>MNSTYSRDQIMSNYLPVIGITMGDAAGVGAEVVVKSLAHASVYAQCRPLVIGDAKRLERANQIVGGEMKIRRIEDASEARYEQGTIDCIDLGLIPDDLPFGQLSAIAGDAAYQYIKRAVELAQSGKIDAICTAPLNKEALHAGGHKYPGHTEMLAHLTGVDEVSMMLVAPQLRVIHVTTHIGIIDAIRKIEPGLVQRTIERGNATLVKAGIERPRIGVCGINPHAGENGLFGYGEEEEKIIPAVTLLQERGLDVTGPLPADTLFFRAGR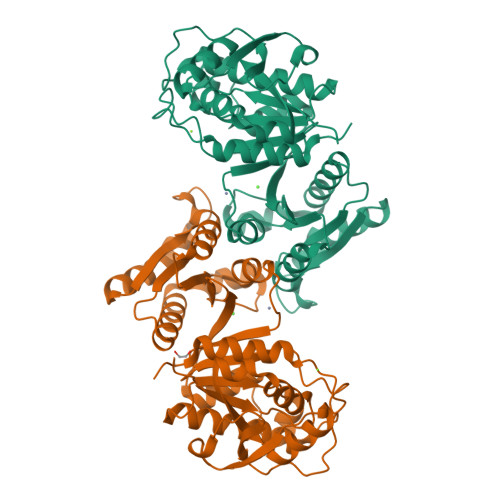GDFDLVVAMYHDQGHGPVKVLGLEAGVNVTVGLEVIRTSVDHGTAFDIAGKGVVDEGSMLEALRQGAELATRR[2x]>MAETEIHTFDDIPMPKLADPLLIYTPANEIFDIASCSAKDIGFAIAHAQIPPGGGPMPHIHYFINEWFWTPEGGIELFHSTKQYPNMDELPVVGGAGRGDLYSIQSEPKQLIYSPNHYMHGFVNPTDKT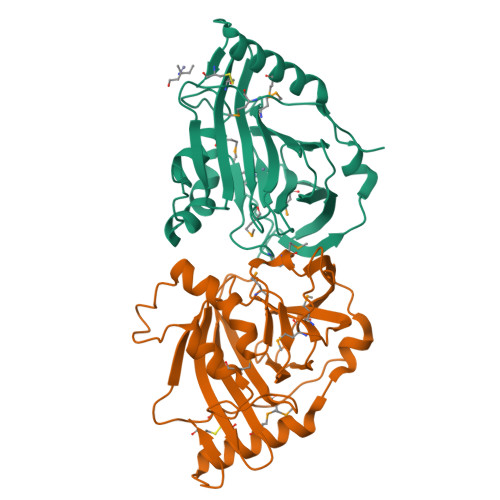LPIVFVWMRNEVAPDFPYHDGGMREYFQAVGPRITDLNNLPELTNAQRAAFASEAPKYGINQSSYFMEYVNTISDKLPAQIAKLKNDKDLERMVEVIEAFNRGDKSVTCS[2x]The T5 family of viruses are tailed bacteriophages characterized by a long non-contractile tail. The bacteriophage DT57C is closely related to the paradigmal T5 phage, though it recognizes a different receptor (BtuB) and features highly divergent lateral tail fibers (LTF). We present a composite map determined by electron cryo-microscopy (cryo-EM) at resolutions ranging between 2.9 Å to 4.9 Å of the entire T5-like phage particle DT57C, and atomic models comprising its core structural proteins. Our results provide a complete atomic structure of a T5-like phage, provide insights into the process of DNA ejection as well as a structural basis for the design of engineered phages and future mechanistic studies.

Finally, DIII comprises two fibronectin type III subdomains, which serve as connection sites for the central tail fiber protein (CFP). To obtain a reconstruction of the CFP region, we re-extracted particles after shifting the center of the reconstruction towards the capsid-distal region of the tail tip complex and performed a refinement with local angular searches. Even though the resulting reconstruction did not allow de novo building of the CFP protein due to the high flexibility of the region, it accommodated well a predicted structural model (see Methods section). The CFP trimer is connected to the TTHP with its own fibronectin domains. Being separated at the proximal part, the CFP monomers merge together as they extend away from the core of the tail tip complex, forming a straight fiber with high β-strand content in a 3-fold symmetric arrangement.

> MISNNAPAKMVLNSIMTGYTLAYVQHSIYTDYDVIGRSFWLKVEESIDRRDYTGVDTFFVMINNLTPSTSYEIQGAFYDSIIDSELLEAKIGINLSNETNFRTKEKPIIVAARSESEPVDVGVGAPIVVVETTGEASYCTIELKSTASEDSEWVKYYIGALGPTIKFGGVPVGDYKIRISGQVTMPDGVTVDSSGYYEYPSVFTVAYNFVPPTAPTNIAFKAARIADGKERYDARIEWDWERGAGANVREFLVTYINSEEYARTGWAKAQKINVGAARAATIISFPWKVEHTFKVSSIAWGPNRQDITESAPATFILNEDTPLDNSFVNETGIDVNYAFIKGSMKEGEIWKQTFLIDAATGAINIGLLDEEGKAPISFDPINRVVNVDGKVITRDINAANFIMTNLSGEDNPAIYTQGKSWGDNNSGIWMGMDNTSAKAKLDIGNATQWIRYDGDVLRISSGVVIGTPNGDVDLGTGMQGKQTVFVYKLATSLPAKPLEQDYPPPGWSKTPPNRTDMTQNIYATTGTLDPVTNRLLEGTSWSDVVQWSGTEGTIGHDGQRGPGMYSVGIAGLGGWDDGQANSFFTSNFSSAPVKYDVLTEYKSDAPGTAFTRQWNGSGWVNPAMVLHGNMIVNGTITADKIVAGNAFLSQIGVNTIYDRAAALSGNPEAQYKMKIDLVNGYIHIR>[3x]DPMQTKYQYGIYIGRFQPFHLGHLRTLNLALEKAEQVIIILGSHRVAADTRNPWRSPERMAMIEACLSPQILKRVHFLTVRDWLYSDNLWLAAVQQ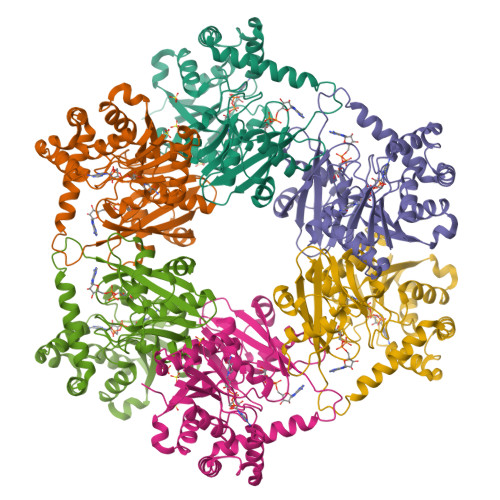QVLKITGGSNSVVVLGHRKDASSYYLNLFPQWDYLETGHYPDFSSTAIRGAYFEGKEGDYLDKVPPAIADYLQTFQKSERYIALCDEYQFLQAYKQAWATAPYAPTFITTDAVVVQAGHVLMVRRQAKPGLGLIALPGGFIKQNETLVEGMLRELKEETRLKVPLPVLRGSIVDSHVFDAPGRSLRGRTITHAYFIQLPGGELPAVKGGDDAQKAWWMSLADLYAQEEQIYEDHFQIIQHFVSKV> MPKYTLPTRDALLKAMQVGETSIEAAEYMATRFEQILTKAKLLPECNDMLEKIKEYAQFVKFKLLSSAQVWSGQERPTSDYQNTQENKAEFLASHLEGLPSGLKLEVAIGDDAKILRGFSSNGKMVEGDQLKTMDGLLEGWLAKNSLAISGGAVVKIDNTGNQTKVDPQEIRQLINDSEKGVAK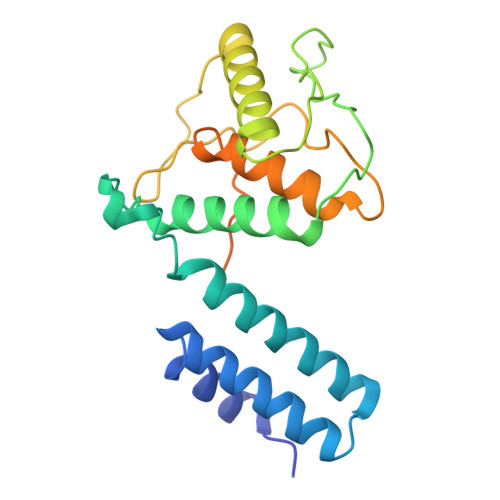YFADKGVGMEVAQRTYQEPKALETKREEIRQEIESGAEAPTTQSIR> MLLGGFVPRRFSQFNRDPCWMFFIFSVGFWLGEY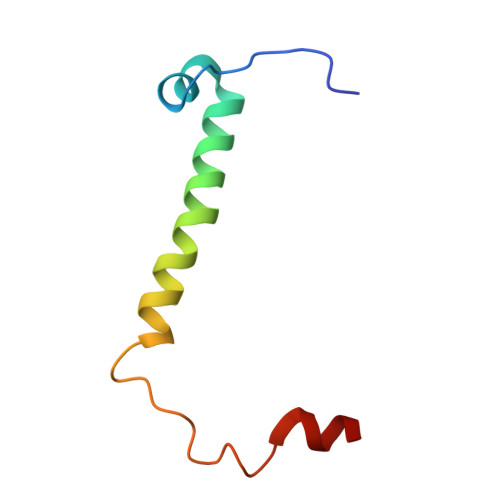PAMMIKYNARDLVYDPHRYVWSHHDDHH>[4x]MGGEIITL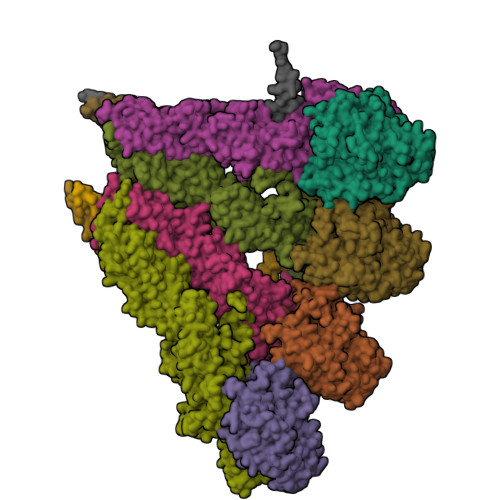QAGQCGNHVGKFLWSQLAKEHAIGTDGLSQLPDSSTERDDDTKPFFRENCRNKFTPRAIMMDSEPSVIADVENTFRGFFDPRNTWVASDGASAGNSWANGYDIGTRNQDDILNKIDKEIDSTDNFEGFQLLHSVAGGTGSGLGSNLLEALCDRYPKKILTTYSVFPARSSEVVVQSYNTILALRRLIEDSDATVVFDNASLLNISGKVFRNPNIDLQHTNQLISTIISSVTNSIRFPSYMYSSMSSIYSTLIPSPELHFLSPSFTPFTSDYIHDDIAHKCHSSYDVMLDLLDPSNSLVSTAMNNPTYFNVYNTIIGNVEPRQISRAMTKLQQRIKFPSWSSSAMHVNIGRRSPYLPLQPNENEVSGMMLSNMSTVVNVFENACNTFDKVFAKGAFLNNYNVGDLFQSMQNVQDEFAESREVVQSLMEDYVAAEQDSYLDDVLVDDENMVGELEEDLDADGDHKLV;>[2x]MEIKEVDDRAELLRYTNNIPLLGKLVNHQPLWSTNPKLKSFSLEKISAPDQRRVQEALVVKDLLNVLIGLEGTYIRYFNDYEPSDPETPIEFKIAKKMDPSFKTFSRRIVRYGKQYMILTRAYEKWSDTSFGMVLQRFAYEIRRFLEDVYLKTLVERLERDFNKVPNFSIRELEQIINETEVNKQMELLYNIYEEIFREIEERRTNQSSQEDFNNFMDSMKNESSLHLRLMVAFDTTVYPVPKGGAILKIFQQKILENLGDRSSVMFLKKLLNNISQDYCTMLYEWLTQGILNDPYQEFMTYDDLEGKTDNIFDTRDRAWDTQYFIRKDVLLRDCDSEEDKNLLFKMLRTGILLKVVRASLQIPTIPSNSSDITIQEINDFADLMEGSNLELYVDKCYSRANEIFLKLFFQGYDLINVLKHLQQIFLGYQSGHNVLKFLTKNMGELTKHYRNDNNANYDKLLQNFELERQSENPNNLMRQLLMIQFDTETLPQVLSHYLQIYPEVPENNSANDDSDPLMHANNFKNMNAILFDELSKERTGAYHGSNLELYTPKSAIYHLKFDINIPYPLNIIISRTCMIKYQIILRYQLVLQYHSRLLDETWMDLNKTPSWKYRGYSHTVKRRIVRATRVLHAKMNHFIKTIMEYFNQNVIDKEVYSLEKCYRNPTLAVAIQNELEGGLTNIMTNRCLSDLIPLQLQIFDIVYKFCKFIKSMRAKLCQLDPVLYEKHKSGMMKTLNEGYRTNNGGQEDVGYQEDAALELIQKLIEYISNASSIFRKCLINFTQELSTEKFDFYDSSSVDAAGIERVLYSIVPPRSASASSQR;>MELEPTLFGIIEALAPQLLSQSHLQTFVSDVVNLLRSSTKSATQLGPLIDFYKLQSLDSPETTIMWHKIEKFLDALFGIQNTDDMVKYLSVFQSLLPSNYRAKIVQKSSGLNMENLANHEHLLSPVRAPSIYTEASFENMDRFSERRSMVSSPNRYVPSSTYSSVTLRQLSNPYYVNTIPEEDILKYVSYTLLATTSALFPFDHEQIQIPSKIPNFESGLLHLIFEAGLLYQSLGYKVEKFRMLNISPMKKALIIEISEELQNYTAFVNNLVSSGTVVSLKSLYREIYENIIRLRIYCRFTEHLEELSGDTFLIELNIFKSHGDLTIRKIATNLFNSMISLYYEYLMNWLTKGLLRATYGEFFIAENTDTNGTDDDFIYHIPIEFNQERVPAFIPKELAYKIFMIGKSYIFLEKYCKEVQWTNEFSKKYHVLYQSNSYRGISTNFFEIINDQYSEIVNHTNQILNQKFHYRDVVFALKNILLMGKSDFMDALIEKANDILATPSDSLPNYKLTRVLQEAVQLSSLRHLMNSPRNSSVINGLDARVLDLGHGSVGWDVFTLDYILYPPLSLVLNVNRPFGRKEYLRIFNFLWRFKKNNYFYQKEMLKSNDIIRSFKKIRGYNPLIRDIINKLSRISILRTQFQQFNSKMESYYLNCIIEENFKEMTRKLQRTENKSQNQFDLIRLNNGTIELNGILTPKAEVLTKSSSSKPQKHAIEKTLNIDELESVHNTFLTNILSHKLFATNTSEISVGDYSGQPYPTSLVLLLNSVYEFVKVYCNLNDIGYEIFIKMNLNDHEASNGLLGKFNTNLKEIVSQYKNFKDRLYIFRADLKNDGDEELFLLSKSLR[2x];>[4x]MDEASHLPNGSLKNMEFTPVGFIKSKRNTTQTQVVSPTKVPNANNGDENEGPVKKRQRRSIDDTIDSTRLFSEASQFDDSFPEIKANIPPSPRSGNVDKSRKRNLIDDLKKDVPMSQPLKEQEVREHQMKKERFDRALESKLLGKRHITYANSDISNKELYINEIKSLKHEIKELRKEKNDTLNNYDTLEEETDDLKNRLQALEKELDAKNKIVNSRKVD>AEAGITGTWSNQLGSTFIVTAGADGALTGTYES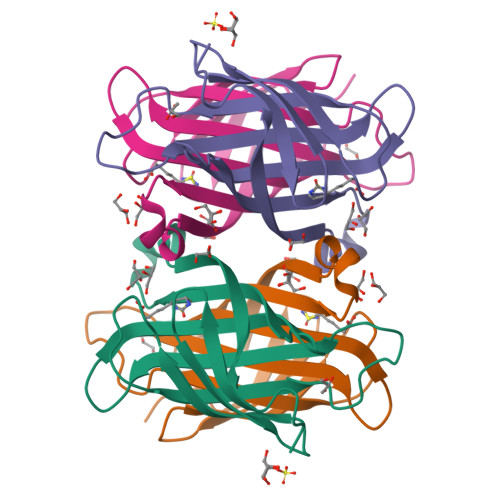AVGNAESRYVLTGRYDSAPATDGSGTALGWTVAWKNNSKNAHSATTWSGQYVGGADAKINTQWLLTSGTTNANAWKSTLVGHDTFTKVKPSAAS[2x]>[4x]GAMTEQQKLTFTALQQRLDSLMLRDRLRFSRRLHGVKKVKNPDAQQAIFQEMAKEIDQAAGKVLLREAARPEITYPDNLPVSQKKQDILEAIRDHQVVIVAGETGSGKTTQLPKICMELGRGIKGLIGHTQPRRLAARTVANRIAEELKTEPGGCIGYKVRFSDHVSDNTMVKLMTDGILLAEIQQDRLLMQYDTIIIDEAHERSLNIDFLLGYLKELLPRRPDLKIIITSATIDPERFSRHFNNAPIIEVSGRTYPVEVRYRPIVEEADDTERDQLQAIFDAVDELSQESHGDILIFMSGEREIRDTADALNKLNLRHTEILPLYARLSNSEQNRVFQSHSGRRIVLATNVAETSLTVPGIKYVIDPGTARISRYSYRTKVQRLPIEPISQASANQRKGRCGRVSEGI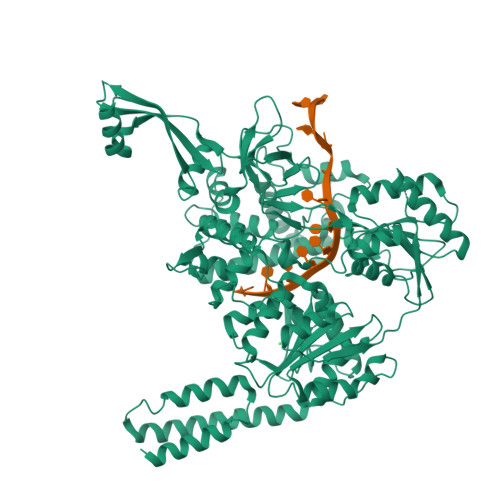CIRLYSEDDFLSRPEFTDPEILRTNLASVILQMTALGLGDIAAFPFVEAPDKRNIQDGVRLLEELGAITTDEQASAYKLTPLGRQLSQLPVDPRLARMVLEAQKHGCVREAMIITSALSIQDPRERPMDKQQASDEKHRRFHDKESDFLAFVNLWNYLGEQQKALSSNAFRRLCRTDYLNYLRVREWQDIYTQLRQVVKELGIPVNSEPAEYREIHIALLTGLLSHIGMKDADKQEYTGARNARFSIFPGSGLFKKPPKWVMVAELVETSRLWGRIAARIDPEWVEPVAQHLIKRTYSEPHWERAQGAVMATEKVTVYGLPIVAARKVNYSQIDPALCRELFIRHALVEGDWQTRHAFFRENLKLRAEVEELEHKS>MEEKEILWNEAKAFIAACYQELGKAAEVKDRLADIKSEIDLTGSYVHTKEELEHGAKMAWRNSNRCIGRLFWNSLNVIDRRDVRTKEEVRDALFHHIETATNNGKIRPTITIFPPEEKGEKQVEIWNHQLIRYAGYESDGERIGDPASCSLTAACEELGWRGERTDFDLLPLIFRMKGDEQPVWYELPRSLVIEVPITHPDIEAFSDLELKWYGVPIISDMKLEVGGIHYNAAPFNGWYMGTEIGARNL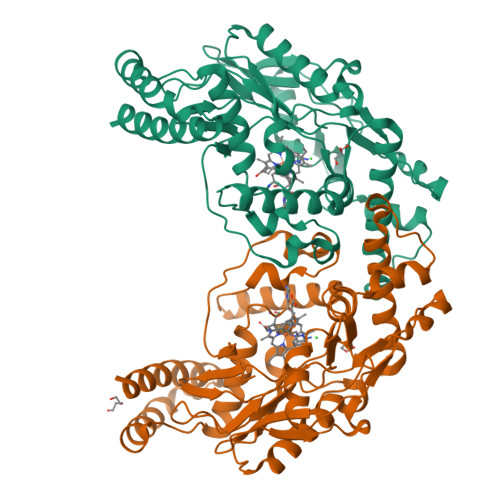ADEKRYDKLKKVASVIGIAADYNTDLWKDQALVELNKAVLHSYKKQGVSIVDHHTAASQFKRFEEQAEEAGRKLTGDWTWLIPPISPAATHIFHRSYDNSIVKPNYFYQDKPYE[2x]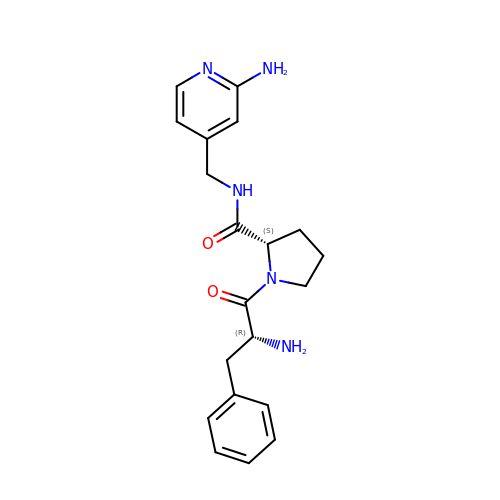(2~{S})-1-[(2~{R})-2-azanyl-3-phenyl-propanoyl]-~{N}-[(2-azanylpyridin-4-yl)methyl]pyrrolidine-2-carboxamide | C20 H25 N5 O2 | LOSWCWUZWRHVLI-SJORKVTESA-N>MSAKNNTHHFPKLLILVGAPGSGKSTFARYFIRTEDNWVRVNRDDFRLMQFGDSLMSPFYEERITKMVEASVIALLKNRTNVIIDATNSSLRSLQDMVHTYTEYADISFKVFDLPVEELVKRCDKRCEQTGKFIPKSAIEKHVTQLQYTKEKFDFKPIPRALKETSLTYADQDTSLPKAVICDLDGTLSLLNGRDPYNASTADQDLLNTPVAMVLKMAKQQGYKVILLSGRENAYREPTERFLAKYQIDYDLLLMRDTNDYRKDNIIKKELFLEEIQGKYFVEFLLDDRNQVVDMWRRELALPCFQVNYGDF[2x];>MEDKTLIKKRIDWFCKNKINAFSPTISPAPKSVERNEIESLYEGILWFVLNGVKEIVIEKKYMGSYCDIYLHRRLEDTYLVSRNGYKINHLDQEQCLRALQGLHDRFSWDGVELRIIQSELMPWSILGKGLINNEFSAYYISHEIHAEYLVQSSLYEKLQKIQQEPAYLSFVADAKVLSAKELKDKYPMHIIRQYQSIRDFKFLDLPHYQQNIQLFKRQLDIFGKEAAPFFKPFNILKEVYTDGREHFVNDNLSFQQINDDDFLHYQFADREDFEAKYPQIRAWVDQVNQSDEEGVVIKPRTAFLPGMPPAFKVRNNDYLTLVYGVDFQDRLQEQIAKRNIKGKLRCSINDWAINAKLLAIPYSELGEENYELKNLVLDRILGEEIENQLDSRL[2x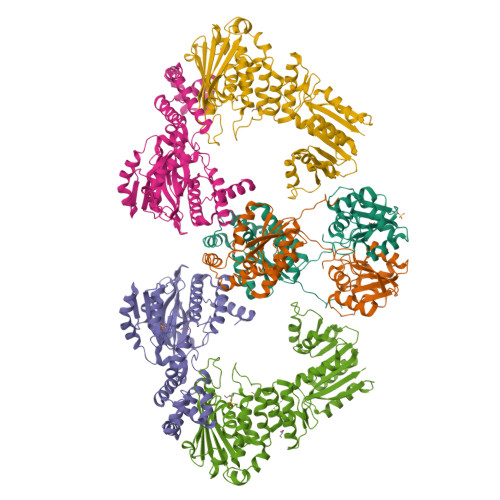];>[2x]MILQIHSQNPHLLDLLNKNPHTDLGIYAKSLRNGQLIGNAVSAYQYDVVFQDTRYSYLPEESNQIDFQSYCSPLVILHICNEFFKELLQEKQTYWSQQIKWLERTRAEVDTYPCTIEVKNLYANSTWYSKGHFMMERYFKNIHITPIVGNNLSLRVEGKSVFEAMNLLSFIAVTTHITNTYGEYTYIDDHFAQKYARILTNIPQVPYFVFYLFIKRAIKSERQFAEIKPMFEAYFKEEGLDIDFQFTDTHGSRMDFIVKELGMEYPILDIGCGELKYYRRFMRRNYNYSHPYFATDTDKSVGDYAALLKERMEADNLYFFSDWTDYEYKNPVNIILTEVIEHNTPEAAEALVKHCLSLNFHKMIITTPNSLFNKYYFDEDPESLRHEDHHFEWTPQEFQDFIRHCVGDTSLEVTYCGIGDRINGETPTQAVVITRK>MSEELVPHPNESLPGPRASPREVWKKGGRLLSVLLAVNVLLLACTLISGGAFNKVAVYDTDVF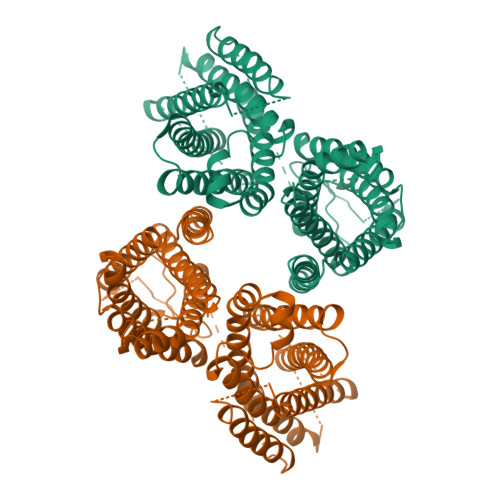ALLTTMMLLAALWIVFYLLRTARCPDAVPYRDAHAGPIWLRGGLVLFGICTLVMDVFKTGYYSSFFECQSAIKILHPIIQAVFVIVQTYFLWISAKDCIHTHLDLTRCGLMFTLATNLAIWMAAVVDESVHQAHSYSGSHGNTSHTRLNPDSKRAGGAAEEDPCLCSTAICQIFQQGYFYLYPFNIEYSLFASTMLYVMWKNVGRLLASTHGHGHTPSRVSLFRETFFAGPVLGLLLFVVGLAVFILYEVQVSGERGHTRQALVIYYSFNIVCLGLMTLVSLSGSVIYRFDRRAMDHHKNPTRTLDVALLMGAALGQYAISYYSIVAVVVGSPRDLQGALNLSHALLMIAQHTFQNVFIIESLHRGPPGAEPREMPPKEPCQGITFANLDAIRTLPSCPPTPRLVIPNLESPQEAVAIISAPRCHWRRRCLKDISLFLLLCNVILWIMPAFGARPHFSNTVEVDFYGYSLWAAIVNICLPFGIFYRMHAVSSLLEVYVLS[2x]> GAIIFSAKDIFEQEFGREVRGYNKVEVDEFLDDVIKDYETYAALVKSLR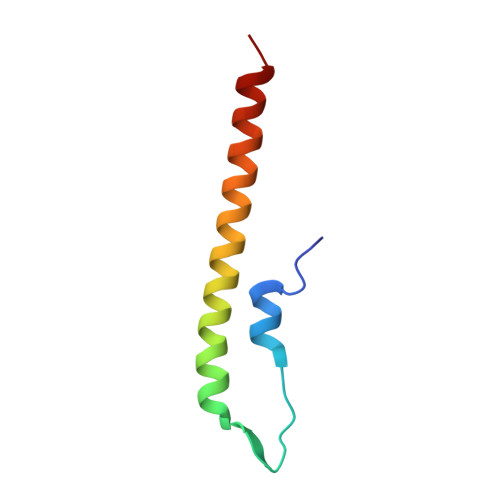QEIADLKEELTRK> MRGSHHHHHHMDYASVAMAAAPTTTTTTNVSLRRQRHRKEKLLVLMGATGTGKSRLSIDLAAHFPLEVINSDKMQVYKGLDITTNKISVPDRGGVPHHLLGEVDPARGELTPADFRSLAGKAVSE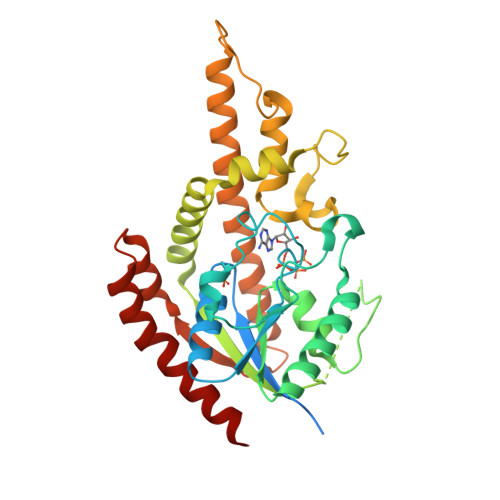ITGRRKLPVLVGGSNSFIHALLVDRFDSSGPGVFEEGSHSVVSSELRYDCCFLWVDVSVKVLTDYLAKRVDDMLELGMFDELAEFYSPEDEDHDEDSATRTGLRKAIGVPEFDRYFEKFRPGDVEGEDPGRDRVRRGAFEEAVRAIKENTCHLAKRQIGKILRLKGAGWDLRRLDATESFRAAMTSDSGEKCTEIWEKQVLEPSVKIVSRFLDE> MVSVSEIRKAQRAEGPATILAIGTANPANCVEQSTYPDFYFKITNSEHKTELKEKFQRMCDKSMIKRRYMYLTEEILKENPNVCEYMAPSLDARQDMVVVEVPRLGKEAAVKAIKEWGQPKSKITHLIVCTTSGVDMPGADYQLTKLLGLRPYVKRYMMYQQGCFAGGTVLRLAKDLAENNKGARVLVVCSEVTAVTFRGPSDTHLDS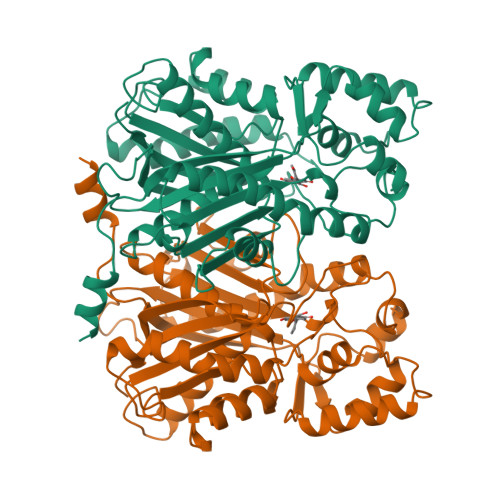LVGQALFGDGAAALIVGSDPVPEIEKPIFEMVWTAQTIAPDSEGAIDGHLREAGLTFHLLKDVPGIVSKNITKALVEAFEPLGISDYNSIFWIAHPGGPAILDQVEQKLALKPEKMNATREVLSEYGNMSSACVLFILDEMRKKSTQNGLKTTGEGLEWGVLFGFGPGLTIETVVLRSVAI3-deoxy-alpha-D-erythro-hex-2-ulofuranosonic 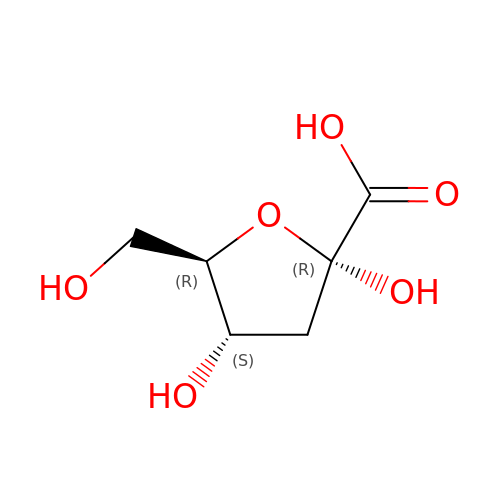acid | C6 H10 O6 | RCUMQJPRQWRUNN-MRKVFDINSA-N> MGSQVSTQRSGSHENSNSATEGSTINYTTINYYKDSYAATAGKQSLKQD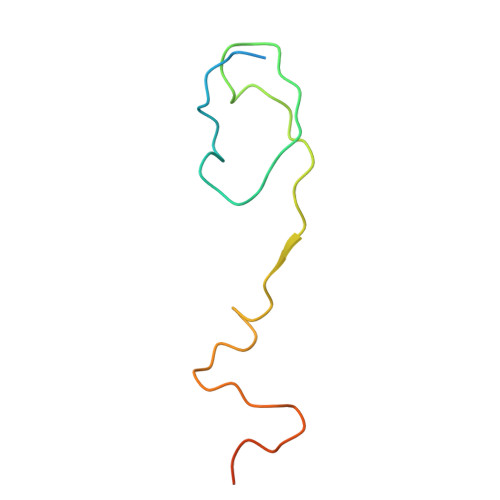PDKFANPVKDIFTEMAAPLKSPSAEACGY>MKLLKILSLVCLSISIGACAEHSMSRAKTSTIPQVNNSIIDQNVQALFNEISADAVFVTYDGQNIKKYGTHLDRAKTAYIPASTFKIANALIGLENHKATSTEIFKWDGKPRFFKAWDKDFTLGEAMQASTVPVYQELARRIGPSLMQSELQRIGYGNMQIGTEVDQFWLKGPLTITPIQEVKFVYDLAQGQLPFKPEVQQQVKEMLYVERRGENRLYAKSGWGMAVDPQVGWYVGFVEKAD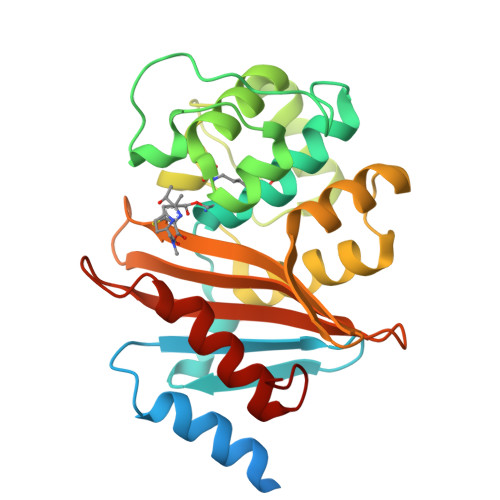GQVVAFALNMQMKAGDDIALRKQLSLDVLDKLGVFHYL[4x]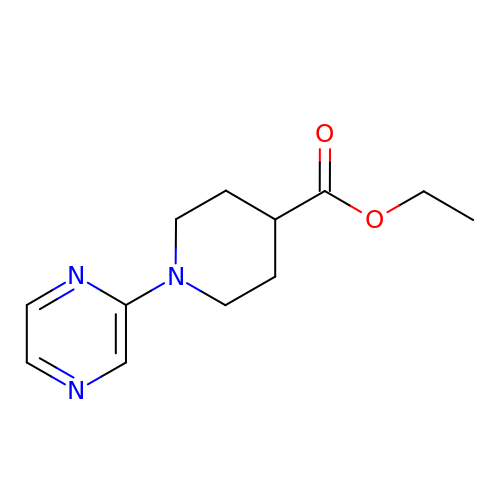ethyl 1-pyrazin-2-ylpiperidine-4-carboxylate | C12 H17 N3 O2 | QYHCUDIPSWPYON-UHFFFAOYSA-N> MHHHHHHSSGRENLYFQGMSDTWSSIQAHKKQLDSLRERLQRRRKQDSGHLDLRNPEAALSPTFRSDSPVPTAPTSGGPKPSTASAVPELATDPELEKKLLHHLSDLALTLPTDAVSICLAISTPDAPATQDGVESLLQKFAAQELIEVKRGLLQDDAHPTLVTYADHSKLSAMM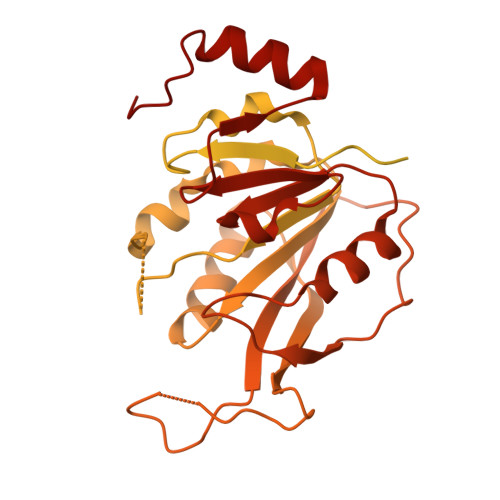GAVAEKKGPGEVAGTVTGQKRRAEQDSTTVAAFASSLVSGLNSSASEPAKEPAKKSRKHAASDVDLEIESLLNQQSTKEQQSKKVSQEILELLNTTTAKEQSIVEKFRSRGRAQVQEFCDYGTKEECMKASDADRPCRKLHFRRIINKHTDESLGDCSFLNTCFHMDTCKYVHYEIDACMDSEAPGSKDHTPSQELALTQSVGGDSSADRLFPPQWICCDIRYLDVSILGKFAVVMADPPWDIHMELPYGTLTDDEMRRLNIPVLQDDGFLFLWVTGRAMELGRECLNLWGYERVDEIIWVKTNQLQRIIRTGRTGHWLNHGKEHCLVGVKGNPQGFNQGLDCDVIVAEVRSTSHKPDEIYGMIERLSPGTRKIELFGRPHNVQPNWITLGNQLDGIHLLDPDVVARFKQKYPDGIISKPKNL>[2x]HHHHHHSSGLVPRGSHMAKSPELDRVIGMIRERAATPRKTTDDDRRLYETMLGSMPLDDDIQTERLGVN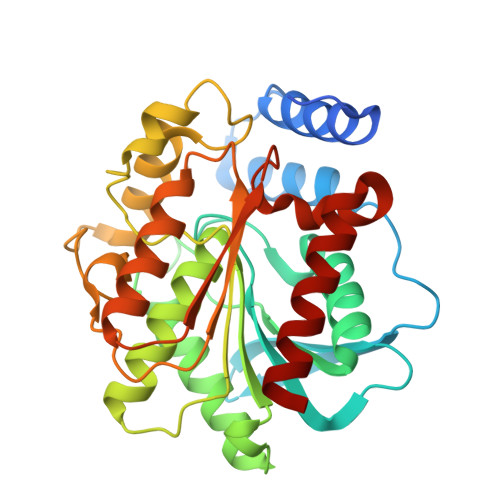GVPAEWIYAPGARDDQVFLYLHGGGYVIGSMRTHRVMLSHIARAAGCRVLGLDYRLAPETPFPAPVEDTVAAYRWLLAHGYDPSRIALGGDSAGGGLVVAALVALRYIGEPLPAAGVCLSPWIDMEATGESFTTNATMDPSVNKERVMWFAALYLGGKNPQAPLASPLYADLQGLPPLLVQVGGIETLLDDARALTTRAKAAGVDADLEVWDDMPHVWQHFAPILPEGKQAIARIGEFLRKQIG>[4x]MRGSHHHHHHGMASMRILLSNDDGVHAPGIQTLAKALREFADVQVVAPDRNRSGASNSL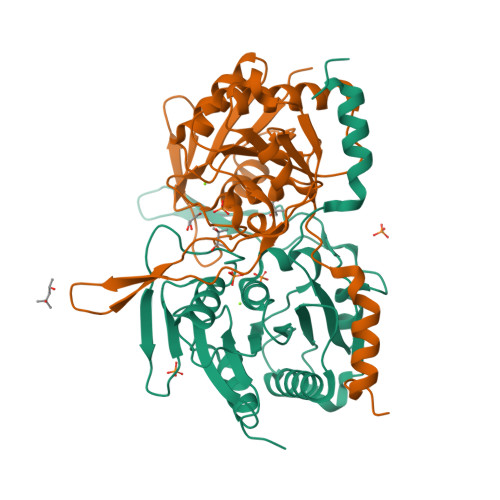TLESSLRTFTFDNGDIAVQMGTPTDCVYLGVNALMRPRPDIVVSGINAGPNLGDDVIYSGTVAAAMAGRHLGFPALAVSLNGYQHYDTAAAVTCALLRGLSREPLRTGRILNVNVPDLPLAQVKGIRVTRCGSRHPADKVIPQEDPRGNTLYWIGPPGDKYDAGPDTDFAAVDEGYVSVTPLHVDLTAHSAHDVVSDWLDSVGVGTQW>MAHHHHHHVTRVLAVANQKGGVAKTTTVASIGAALTEQGRRVLLVDLDPQGCLTFSLGHDPDKLPVSVHEVLLGDVEPSAALV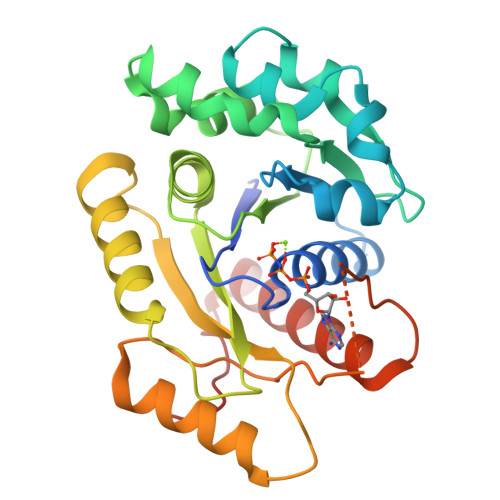RTDEGMTLLPANIDLAGAEAMLLMRAGREYALKRALAKLDGDFDVVIIDCPPSLGVLTLNGLTAAHDVIVPLQCETLAHRGVGQFLRTISDVQQITNPDLKLLGALPTLYDSRTTHSRDVLLDVADRYELPVLAPPIPRTVRFAEASASGSSVLAGRKSKGAIAYREFADALLRHWKSGRKMPTFTPEVV[2x]(2R,4S)-2-[(1R)-1-{[(2R)-2-carboxy-2-(thiophen-3-yl)acetyl]amino}-2-oxoethyl]-5,5-dimethyl-1,3-thiazolidine-4-carboxylic 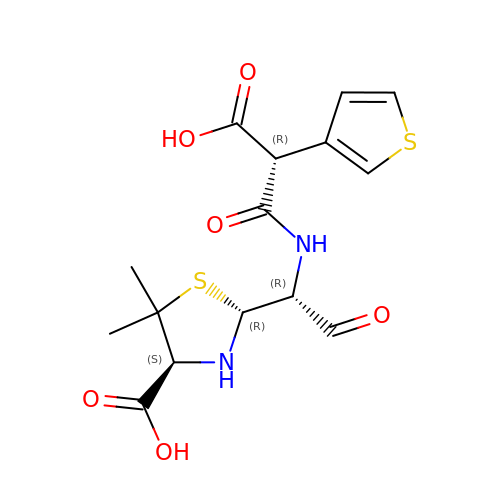acid | C15 H18 N2 O6 S2 | GQZADNJRZOHJDT-MWGHHZFTSA-N> GSMSLKPFTYPFPETRFLHAGPNVYKFKIRYGKSIRGEEIENKEVITQELEDSVRVVLGNLDNLQPFATEHFIVFPYKSKWERVSHLK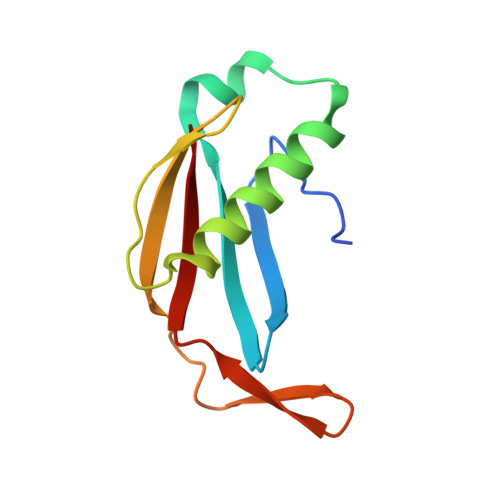FKHGEIILIPYPFVFTLYVE> ACRPGATRMKWYFQKPYVRRVKSDFFRFPLLSQVTKQKIDWQYHHPRSGYEAACIFGPNTLEVTNLPMGKTCQYLQERLWRFFGKFGIVEQVRVLPHERDPYQTCGTAYVCFRSRMASLRAVRLPVHLPASLHNRVLHLRHLGTDRTSDDLFYFRRQQAISNLVAIAQQLYAYLEERGPLPAHRALRLLFERSYPRLAWRQAGVSVRTCCGSWLGFFSRSPFNELFYLAREDEVARPTEVTELEADPRASRKMISNEGTEGAAETRGRKTKSKLGDTKDGTSPGLKSLTDREENAMLEKMVIFPHLLSREKLQALLLRAGRLLQMDLQNELSVHWRTDRPPLPDWTQKQIQLWQHQDPLPEELQIWSRTKDYYKIHEERFLFKLKLKKERAQAKQEMKQQRRRLE;> GADHVFNIFKDLPDHKILEDKHYPAWLFTLDKPEKTYGELAMTFLYGVGIENATLDEYLRFTRLHTKNLIKLNNMRLKKSKRSSVKPLFWDA;> GGPGRALCTPTFHGLSDGPYRRLKFSLKPIRHDYRDVLVSADLRKLAETAQELLRGKETKRRAFWEIFSKRVKASAHMLSPSLMALIAKSFDVHDRDTGIYVALATVLPEAVKRADGRSLLTLSDVFSRRLKRDSNPHLFSTLARQLPNALYQLTGKDVLRILSSLDAAGLADMLACRQVARKLLAELDELDSVDLADASAVFASQGYRNPELYSALARRAVDVKDSFDAPTVFRLLSGFSQNAVACDELLESFSTLLVSSKDQFTQHER;> KNFKTDLIRMQWPAMRDEMVRFFQSQNAIAFDKISKRHPSASLSSDASSSSSSPSANRGERRATAEEVDREEQGKLSFAEMVVGSTRSACGVLGAGRSSAVDVACKPWKRFVRKEDIQRAGYVPCIVEKYGIERRLAIHRDTLEALAFDEQHGHLSYLFQARLFRLRIGNWIEECIPTFVQADPVARRLYFVKFERHVAGKISEVDIPTTMVGLLACPAYQRGYHVELVMPTIRCQCVGAEIPPPFFVDVSRLHYSPPYTAITLQDLQHLLPADGSARFHPSYDAATQEVAWAYEVGSLPDAPLPADYVDPNFVDRKGQKMDVCFRNHFPN;> PSPSSFPHYSRRHFKRQSPRQLHQLASNLAARGCTDVVLWSSMIQRAIEVNRSPESGAADVSVAPFRFFEALGFLGAVSSLGLTDRELFLSFVPCFLRSLSALEPRHLVQLLTVYEAAGVRPRGLYVAVFNRVLKLAPSFYSHEFADFLCCLARLKIANPSFLSAFSQTLVSRLPEIAFPDACRCVGALRSLGVAQQSLFDLFDERQKKELELLPTQLLLEDFQKVLSLEFSWQAYENMIQEEFIKRTEAMIDDKDVDELADPFACLNFMKTRNLVSDKFLLALSKWCRAAVNRPATRSYKRPLAHQLVELHDLMRERNLEQNKALEQAVLRFVADDGGCKRRPREVKPLLYQRNRRYISCPDLIPDGIEPARPCAEALPDVFMERQASLVRACTPEDLARQELPFAVQAETAYRRLQRNKRFLRFVQEE;> RWRPKKSYKKRTMGLPSTKARRRWAQMRRG;> GKRYIPFRTPRNPKSKHILATPPPLFAATALDARSFVWPPLHFVERRRRLLMEKNLL;> GLWRQSIVRCADNTGVIKACIIGIRNKYGTGKIGARIRVSVRDKTPECTAPKMPKGVIVRRRKETRRKDGSYIKFDENAFVIIQKNKARGTKIKGPVPMEIRHNCKTLARWIFA;> GWSKVVNFLNKGVQRRPHRRLPGQPHHQWNMLKTQLDQLVRSDRLELTLPRAHELQQYAEELVHFAKQNTPESSLIVESMIFTPAARRKLFHELCPLYANRPFFYTRVVNQHRLRMRDAAPMAYLEFVDRPGEIRPARPVGFERKQAIWEEMQATRRGRRQWWNHAKKLGLIDEETGDVISDINALRRPSAAEWEESDSEEEKADSPSPYKMVAAPKRALEPFFVDLPPPTERYRKQRYVFKRFRP;> MTTREYEEAFLPRRLKRIKVFNTPPPSELPAFFHKRLDNAHSNPRSILKLYRQYMRKDDYPAYDWLVRCFCHLGNVFGFNSFWATKDKQVIQALPSFKFLVYDLIERKHLIEARQVPRLLYAFACLEYRSWHLLPTLLEHVEANLEKWRTPTLANMALTLALLGVGDDAPDHNQFGPPDLLSRDYTGLVSKLALEVHRRLLALQSASSSGPRKSPLHDSLGCMPFDYAGLAFALTLQGSYDLCLPSDETAKSTLALFLQRACEPLSLEQLENSGWVQFFLYQTLYCVDVEKPKREVEVKKAVPFAFQKHLHLSWLDKILINAQPQGNELLQLDVDAALKRLHITDALINCSAGRQWDEQHCWFAGHLVRSRNLALEYDYLLPLGPGRPKVSGWLACKRRMLKAFGLNVATIHQSFWSLLNLEQKDVQLTRLLAQFPPVLEAVKDEKKAYEEDRHLRFQRHARQKFETWPPEKLEI;> SQSYPKGSFHEGHINPFADVQWISRPFMKRNMPRDHHPLAKQHTSLKAVTMLDEESGNHWHVLDGKGRSVGGLAAQVVRLLQGKHRVDFTPRTAAGDSVIVVNAIHLKMAGHTWDTKVYKFDRKTHPAGPKIITAKTIMARNPAMILNLAVKRMLPPNRLRPIMYRKLFVYAGALHPHWQVPQVIVPAKTPAEVSFLPFSVERADPVQAAARIAALG;> MQIPRDVIFEVVRGFRGRSRNCIKIARVRAMKALLYSYIMRRQRQRRYRVFWIGRINAAGREWSFPYAWLATSLWRQNIWLDRKMLANLAETEPASFRALVNEGKSVYFWNPDKVRDIQDL;> VRPNQGRNDYNQVGGKKRGQGVQVLPETIRLLIETRKAATAGGPVGRQPLPKATEATGVSSWGRDRRFPITEALRLPTVAEVNAPWEPYDETANKRRSGSRPLSSSVDGCHENHDPSSDGVARGQDRLGRLDKVVLHSGDISRLRVDATVVGAVRSFKTVGDGRGFTGCSALLEGAGPFLSSFVSQQRRHLGEELLHTPVRGDPSSAQTVAAAAVRGLRRGIHHFTASTVPLPLRSSSTVPSLAEVEEMPIMELSQLAARAALLGSARGGGTRGFGLSSHPQTRRLEGVSTASGATEGSDAALSFANEVRDQATASQFPARDLIQTPLDPSQLSPPGAVLISPGFNLPSNFLIHVAEPNAVLSNQQMLDTLFRLEEREALRRKEQLLSRFGAAQAADEAMSDDEVREEDNEMTPRSMWQDDAERDTGVQRMLLLEECYINALNAAWALGVRSVALPCLGAGVGRFPVYIAARCAARGVARWMSEHRDCDAWENAESDKRADFDRIVFCTSSDVEWNALRRVIPQFLS;> GTSRRLSLFFSDPPPAYALSLHAGYKIQAALCVDRLPLVYREPRYEKRWREFKEQWEAQTKNGLTLADEITFMKFPFHFFETEEAQKKREELISKTGDAEVSELELLLSEEGFSGKRKLQRDRDAKKAAREEQSAVKSAGRGQDEKGLRSLEREPERTLYLIVRYGDSWQFPLEDRIHGQSMRSTLKRLCSEQLGSSYAPFLLGYSPFSYAKRTYPKKTKEAGILGRKIFYYRAHHIPGSENLKLPEGSPVSDFAWVTLQELPAYISPRKLAAVSAGLLLEE;> RWWTRASGMRNPVKWTRDWEVLNRKVYFAFDEREIRRSMLDAVNAHRKTASLFHRMINAVPGVAHAMSLPGPHTFFLPSDKACRDHLSPDSLHALTERVAFLEEQQRQRVGARVQVEGGVSVRGGTAAAIADRVAKTTEQLRTFVLAHLIPGEWRMKTLLLACGAGDPRRNGSLRYQDTDRELFAPVMYASRLGTGEKTKRRQTASREGVEHENAQELGRTRDEETDRSSVFLLPPPQSTDEPLPVWVQASRYAAFLPITTSTNFPRFEGTECRGNSDREEAESVENSGEYSQRRSTVGGALHLWVGGALVTKGDLRAHNGVVHMIDKPLIPVQLLAS;> WHRGTLSLLCSSCRYVVRKWHVPILGVDCNANPRHKQALSVPAPRSRGIPKHLYPFLVGKQYPRHPRWRQAFTHRSRMGKYKPQVARN;> SANPYKPKSREVFHPYVPAPEHLPPPAYTTAVLKPMQQFIPKDFYRDMRVDSLRDGVSLGSDFPWNVTHKYRFWRRRKYNIQLDDRFIRLSPVTGVDYYPRLNVFAVQWREDGQHRIRWFRAAYGLTRAMRAAENFRKTLEATGRVDN;> AISHLNPSISKGKVHYRVPNPYIPVLLLQAVPGLGKRGELKQVRRGTLRLFLAPKGLAVVASWQNIDAFYLAEKEEEERRRRAQAGR;> AKVGPSKGRGPLLAKFAPVGFKKGFGAIGLGRHTKKGFFIINTMLVPMFKVPDLSNCKLKCYVAPDTYRIVQQSFNKRE;> GILRPRERLLLNALKKEADIRYRGRRMHKRFRSWAQQRVRHYWLPQKVCVTSDPQLMDGSYIAACVQKAATLRKHDLQLWHGFSKRILELADSLTPQQMGYIFYGYGKSLFRHEELYRGLLPFVAEALPEFHSHALMTVAWALERVRVNDRAVVAQIAEEALAKKDLMRPADFIKIVNCVARMGAAPPSLAAALSAELMRVLDEKCNALLFRGAVDHVAVATLYSDPLRLYLLERFTKTAICCRPMHYQKAFQSAVAIRVLHPPVWQQLSKAVRNFYIRLSLRRIPQRARRPSPLHWDVSNALAKLGVFHRNTFQWGCFWIDIGEIDDRRQCWFVDGPSDFYSSTNEYTEANKLQHRILSELGWNIRRVRWNDWVQLGTDMDAKVEYLRKLRERPPWPAILTDGPSSSRQEMVANLRSARDVQRALKERREKNRQPHSLVMNL;> SGALQRAVREIPWKSRQDILRERERPVYAAECRGTPRREYSKNVIDGVRVKPTFNPFVKLNKAKRYVLDNWPSRNWDDWSPYRCYVRGSRRRYNIPQDLLPYKDELGEWHPPRLSARYQADVKKQYLMNNLPWVWQKDFYEGKMHFGDREPLGPKVWYRKAFREERVKEAMRKMDDLVLDYRQENRDRRRYNWFEKVVHDFAGEEIATQFIRKRKEPKL;> IATLVERSLEKHKDRLFDCGASGQPVTYKEVAEHARSISETLKAAAAYLHVPLTLPSALGRAGADGQARHTATSTEDCTGSASTLKCRGKPLNRPTIGLIVPPNSVAILAHLVGVWQCGGVGLLLPFPDPACLPFVADSTAAAAASAANAAVLFAKGGKTLHTYRPDALFQGNTGPSVYAKTVNPNSLPFLNSQNNAHNRNGVAQLWEYQAAESRCHLLVVTPEVAPMAAEVASKLSIPICVLRTSWVRKSDGTNGAEEQRAPERDLWSVRGRNKLEVKAYVPEVFHDSSRTSRNITRWQLLEVTPHECTHAAADEESIAEVAAPATHFFQGPAAHAPRAVIYSHKALSDQVIRNKDLLQLNAEDHVVILHLPFFGSHRSGTGSQASSRMLCTPKGLVAVAMPAVAAGSTLSFLSSSDKIQDSLLPLPLQLQRLQDRLPQNEKIPRQPEQRQALLPLGCDIPEKTPWRCSGTTTRGPLVPRGNQEGLQVDFTGAYENTLEVNALQMWEKIASLHEDGRNTTRSRKQRFTSRDKATPELSRQATVLAMDAETAATMVQVIATERFQMEGTNEKAHASGGSDASRFPTITSKDITRYKAAVKSLRLICICTDEGDLGASFSGRWSSSNKGGGIRIQSLLRSLQALAGPDTKILHLCSLTETGLLMVGGPLPDGSPGSRERGEKSDFGEPLQDHLSTGCKDSKTQCLDATDGEDRANFTGVVAPGIKVEIDDETDQLRVRSGHMAMGFHGRPRSTQESFDSAGLFRSSFGGSLVTNRRNDTDIIGCDRGEAEQRVELFKCVYSAAVPRLPLLHRLIASFKNSPKMESHIEGYVKKKPIAGRDWNNLHAPRKHWKKMFL;> SVVGRFRLIVPAATAKPSPAIGQTLGPLGINMMQFCKEFNARTANVRPEVPLQVTIVPLTDRSYKFSIRAPSNIWFLLRTARCPMGSESPGHQSVGNVTLKEIYHIARCKSMDWPLIGMSLRGICRSLIGTARASGIEISKEILPAYHKRDYTDVQALDSMRKDMRQRKKAAKRAAT;> YKPVIDWVKNRINARMRQYRKRSLKKKNHSKVIQRFKLTRFGWQRLRSGRNGEKENLTHKQLKRTMGYTFVSRDDLWKFRFQLPSHILRLRDAPINRNPNIRKIRRSLPSYFG;> MLWLAATHRNRVAFQLFATPREPTASKAAAAARAAAEAVARSSTVSAPFTVQKQQRLLALLAASSSVADPSADLFRVHGLPGFSGFRPSSPPHLSKLFRGRVSRHLSCRRVNHLGRNNSGRITVRFRGAGHFRRLRFVDYKRGRKDIFGTVLRLEYDPNRSAHLALLQYDDGVLSYILATEVTRPGDRVVASKHASIAPGNCLPLGNIPVSTIVHNVELRPGAGGQIVRAGGCYATVVAKDRHFVTLKLSSTEVRRFPADCWATVGQVSNAAHAERIRGKAGVSYWMGERPRTRGKAMNPVDHPHGGGTGKKGLKRPPVSKWGILCKGYKTRAKKKPLGLIVRR;> LPNPLVHLDISIGGRDAGRMVFQLFADTHPITAENFRCLCTGETGLGYWMRPRWYKSTPFHRIVPGFMCQGGDIHRGDGRGGECIYGQFFRDERFLYKHSKRGLLSMAKARRQHTNNSQFFITFDACPWLDGEHVVFGQLQSGAEVLDQIEEQGTPGGWRKRPVEIWNCGELLLNTLREIPREAPAAVRHQEMLKDLIIDATERPEKLYEPSEQVIPIPDDVYIKARRGF;> NKVRTDKKERKRAFPQRGFWKKQNFLQVKNNTVRLAFAVQGVDLLKLKRLRWGEVRKGNTGWWTDDYRSP;> IADRVRTSWTYRHSRYSGGVRFSLPRFMVTKRTYLSTKFRRPSTVTKWGNPQYTLPSNVQREMQENSAEGDTDQATSEELGGRTGKKELGRNGKSAGKTKKAADTAAQEVQHTPKYCDMLFLHQEDQQSRRR;> SRYVKVYRKVMNLQRRKTPLPWTPTFLEFSKEPSVPFPVREKLQPAPIDLSYYLNMEVGDLVEVLHGPDCGRQGVVLSISKKRNTVVVDGCNMKKSFWNPGVGASLITQEMPIHITNVALLDPVVKRPTRVKRRFMMNGECVRISKLSGSAMPEPVSTSALRQPNLYQEYLRQKALGPPLKASYARPDPLHLKILQRLARHISWGQGSPLPTAENPRVNSPEPMALRR;> RSRSKRLFVQLKSAAMTNFCYVTRKSPEKKNFRIALRKYDPGVNKHVMFYEARLPSEKNKKQITLSLQRYIRWTGKQVKLLLDKVEKAWEYGRFQKYFDNQAPLLTDRRGRAVPRYK;> SHVPYKVVRTPSGNLPVYSRVRKHGTEVTTIVRHAFGDITAMKKDLVAICEAPVRERLGTLEVKGLHVLKIKQWLRSLG;> SVASRIHFLNSRTRFQTAVHASDVAPPFLLLPLASPRPLLAYHHRFRTRNRKRGSRFHPHPLPLPPPPLSPPRSDAAHLFAGKPLAASAVSTAAGQQTLPPPLLRHLQGLFPVFRGPECDPSCGVGPAGEAAGLALLPPPSLVEPRHLEDLARRALQARGETRDAASGACKSDRLFWRELAARVEKVRDLLPIESLVRLLTILTLNGASGTVRPVKQIFQAFETQDEDTPATPANRTGLRLASETLPCVRPLPPRLLLASTREFLEDLKKLSPPATAALAATFAWSNCASSALLFALMERWAWRQPRAEPSVQTDVESEVEPLGKRREAETGVEEEAENAKKLEAVETQGHLGDFTPADFALFVSALGHLLSQQEATHVKYSRQARHLREISGKQIMAAFREQKRQKGKQTADANFENFEETKSAWHFTAAFFDGCCRFMATRAESFSLFSFASAARTLVENLDAVALVGEAAESRALAVDGEGAGSVESLGIHGISTFSSFEGSVSRSEKPHVACPTPDSVEALAKAISLFVASWDGGDKTHGRLATRAANLLLVARLLRAASQCELYIHLHRALRLEAEGSGEGKSPQKRNSGEQASGAGVDDGGRGIAVDTVGACKTLLEHISCELGLLHSELEALPLLNSTLEDADDSADEKKAVDAPTERGFVHISPDTVYVRNELLAAAGESAAAVVRLHHAKSLLQATDEVARDSQSLRKGEAENVCHLSTGARVDRVKRWMRGQQAERMQLETLGELKSEAEHLADAIDRVLRERGAAGLPTEQLADLMEVFALCVGDKRVSQTPEETSRWFRLGLGDKAEKMNQANLSSLQALSSEIVRRYAALDVNQKRRIKWATRQMDWKDPYLNHCLGRFTAAVTRQR;> YDSRWVKRLDRLRESKFYDPAPIIKEEEILEADKIHPLLKKVTPSWNSRRTGLLAYKIGMMSLWDGWGERHAVTVCQVDRCVVMDQRTLDKDGYEACVMGIGYKPIHKVTKPMLGVYIRSQIEPKSRIAEFKCSSDCLLPVGHEMSVRHFTPGQQVFVSGWSKDKGYLGVKKRWGFAGQNASHGVEAKAHSSPGSIGQSKTVNVVWRFKKMAGHAGGDPRVVNCKVFRIEAQRNLIFLKGCVPGYKGSLIKISDARGKTHHRHNRHIPLHFPTFVPEPGVSYPVTLECPDAEQDPFLYPEIAIADK;> YWPPTRKDRSKRIRLPSGKKCFVFNAKRDQDGELEPVLCFVDSQDNLLMWFNEEELLEFEKLMPRLESYYELWEEKASRTRMKEAIVAEAES;> SSGLPNTKRRIRDPFWRRSGWWRWRQQEVKAMNRSRAFRRHLFPRFTTETVSFVDAAEAEAKRFKEIVAETGRYPGQTVNFFVPKVEGAKLDPFAALPSRQKRLKLRRKAVREAEEAEKAREDADFVWRGKGGGRVWEERKANIPLGKKKLLLYCTIIKGLQITDAIDWLSSLCLHRVNYLLNLLNASRKKIHEQGGDISRVYVESYMLNIQGQIKRPQFRLRMVNLIKTWKFAVVLRFREYPMDEYFHKLFILKHVPRSLTTDMRLALAGQRVGLHAVRDWYPFLDSKTRFFHRKRLKWLDRTRQFDYCLARRVFKSKYEENCRRRKIQVLQARGASDAVIEEAN;> GNFRIKPPGARHAFPKLGTHRMVMFRRMNLLNWPPEDASPLHPIEPWGRQFFVFNAFATIDPADWCGPRGPFPRLPPLAKPAPDAATLAASPSSLLSALRETEERSATRTVMCVTDFAQRPLMFLGKDDFRALRENLPRIKEELKAFKERIQPNPVHAQYDLRRKLLVYPRQAMQRLKTGEHGGYGTRRGTIRERKT;> PPKTPRNVFFPWQVFSVHRTGAFLERRRVALKVPVNLTKFEIQSYLEKIYGARVLKVSTLIVVPRRRRDIFGPRPSMRYYRVGCTFKKAIVTLEDGVPDAVKMLRSSIELAKNPDITKHNLTYSGRVRAFKPPSAAQRWEMGESKYAWRLPIPNLLAGDEMQLNPALRIDESTTQMFPDFSKPFFHNAHFNFSWKPEEVPFQQTVKLDITPWRR;> FFYYRFHKRIGKGNFNRYLEFYQKPRGIENTLRLRYNYTPTFTAKKRSEMWKVNLVKKIAHATDAKQVLDVWTYYRHRRTKRPYHYLLALQRLVEVGGCDPTDFRFRLIARGIYRTAKRFINLPRVCVYLAKLNATGDLQDLSRFLIPQVEAYFPFQLCLLAHAFGSVRLQDKVLFAAIDEALRPHLSELPAAMLVKLTQGYAGALVHNYGLLARVSLLLQQRLSRAATGEADPLTACDEEDETGRTLSSKEPQGGSRQRETTKAAREITEAEDDCLEATEKKTVKRRHSGPLLPTLHHLLAFGRVCADLKYQDFGYLEMLSIQMQAAFRADLAVSSSRETFQRFSPFSVQELVEIFHRLKVNDVSLLLAALRHVQARMHDYPPSCVASIGFCTAQMLPCDASTVRQVHAQMLEVLQEAVPLLDLCSLGQLAAFAKKAKPRRNRSALRSSVFEAVEARVIELQGDGRTVFDVGRLLELLSLNGRRVSEEAFHILCRQAHRHLDLFEPQDFCRLARALARVKCQGSRGEQSEGLQASSLVNALARRTLRQEDEFSPRDFLSLLRSLTLAGPPDRVYAVPLKEKLRRKQVLHNYFPASQSEDAEAFEDSEQLLESDLPPSSRQTPTLRKGRLLLGPQVIRRPQQQGSPESAEGEARSEKETLEEESLSYSPVPDGEQEAEVNGNHAGKSVSVLSEGGRSRIRRRRLEEKLRIAEEEGWDLLHRRVASLRQLKGWL;> EKLYGIPHNGFWNQRRMYTEARGQTAALAAMQDPVEVLNFAGSNEMASTYLLVSCLRRVSALCDKKHAVLETVAKDERLQRLIQLISPHVDDCDARCLVDLCWAVWGFRGAPDVVEPLLNRMASVVVRRENAFTPKQLGTIAFTFSWFRGAPTDTVADFVLAECVKLLPEMEPFHVTLLFGSLRRMRRLNRDVANLMIEKLTDDIDRFTSDDVVGVLRALAANSITRGFLLRRVATLVFDNLDSFKPKQLASVLNSLTLLRFLTVENGEELFSCLSGSLSELPAASIAEILEALTILNFPRPEVVRTCLDLLAEKNGLISQGSWVRDHMIIAAHAVIQFQLYDKNPVVKPLLEELFRSRVNSSRTQHRVEEVIHALDLEKASPRVDVPPYWRAMIDQANREEQARLEHSGLQNELTLVLDSLRGKFQLQIQKNQQAGPYSVQFLDDETKICIEIDYPCCRTPHIIKARHLKQLGYHYLLVDCWQWRRLRSEAEQTVFLKQLLSGPLLEVGRL;> RLQRLIQLISPHVDDCDARCLVDLCWAVWGFRGAPDVVEPLLNRMASVVVRRENAFTPKQLGTIAFTFSWFRGAPTDTVADFVLAECVKLLPEMEPFHVTLLFGSLRRMRRLNRDVANLMIEKLTDDIDRFTSDDVVGVLRALAANSITRGFLLRRVATLVFDNLDSFKPKQLASVLNSLTLLRFLTVENGEELFSCLSGSLSELPAASIAEILEALTILNFPRPEVVRTCLDLLAEKNGLISQGSWVRDHMIIAAHAVIQFQLYDKNPVVKPLLEELFRSRVNSSRTQHRVEEVIHALDLEKASPRVDVPPYWRAMIDQANREEQARLEHSGLQNELTLVLDSLRGKFQLQIQKNQQAGPYSVQFLDDETKICIEIDYPCCRTPHIIKARHLKQLGYHYLLVDCWQWRRLRSEAEQTVFLKQLLSGPLLEVGRLEG;> RELGLGAASAIEQKASAFFSRLTDVQQRQLEKQGLLASRFYRFLVISLMEKEGTFTYYDFYVWRKGCLAYLKAAEEEMQGIVGKSARKLADLGWEKLRPSTSPEFKEMELHLKILSHFTPEELSRDTAEQFTSAAIKNIAKAAETSVKNVKNVLLGHAIALTDRTWYMRLMEMQRPIPQSVEDYLLLAETDRPYMIRLPYGEKFYNYELEEALAKKRASERHKSQRDVPRLGRKQHRIRRLFVPNARVAFDRWARIPHARLDAYGNFLYRLNQPAKGAAAVARAAEREKLRVEMSENAEFYSDAALSASRITLNNLPPGAFRRRTGMQRKSGEIHHVAPPRDPVLRELFAAAIQREKDEKRNRERRAQEDAAAAEK;> GGSYGYDAFFRGAAEVLNGSNIQLPHLPENEEQKEGKVYQLHSVRFPPQVRRLGANYFFRRQRAVPLTYYHHLVEAKPASEGSAPDGVHAQTGRGQALCFVASANPGYLQSKELENAVFESTRGFACQLILEGRGVKAYFDPEWPNLMVRLGVGVKPLALRRLAEQYATRAKIFVDKRGLLLTVHGYDKCAVGTLAMSLFNHLQANPYTMKGAHVAMHPIKKKVTR;> GIDELWKGSYLDPTIGAKQKEANAVAGDAWPACLLRMKSFEDLHKLWYICLKEKNLLMGERWAARQHKQEMKQPERLQKVRRTMRRILIVLTKREIQQQCLRAKDILAKQQKREALETRRFQLEEKMLQLEHRIRRMEPAQSLQKEAWQATLDRYRSDHEDILIQLHPLRKETTQLLAPDWRYERKYSDLPGPIRWKKQYIPALEDQYRKPIRF;> PLQPSFTPSVAFPAHKPVPLNSPLSPSVHAAPQVRRPGSVVRMNEVIRHWWSVPAVGFNSVLEVPIYRFEVFQRRAEEAGEGEASIAEEGDHPEEEEGCVVLPNDIFGLPLRPDILYRCYWFYRRAIAGWTERMQLFKWEWPGSKRKLRTQQRSGRARIGWRKAPGKYVGVKAHPLRPHDQRIKINKRLLWQGLKIMLSAKFAQGQITVVDHFNLQSHKTKHCVRHLRRLLGRKCPSALLVHEGTTDVNDNFRYATAHILAVRRENVEGINVYNLLKYRQLVITEKALLKLIYNIQTYPEKRGWLPKYATPDGKPAPAPEKVEGWDREWRQMKERERNAKFSKALLRERILKWKWSDETKGAIKVPRVDPFKGFRLARFSLHEPTMPWEKFEENYVDTDPLEDEEDGDMFDEAQALGEETQRLERLDHEELSDAAAYDDMSLTDMPLTERMHRPKRLENFKMEP;> SRSFPLGIKQTLPRHILRATGDQPSSSSSMSALAAKPPKSPCSLSVDTCKDSSPSELVVYERRDGKRWVHRHQLSLYLSHAVGLGYFRAQFEDSSVTPAAVFDCLSHLVRPPVHAARSEEDEGDEGGERRQNKQVDGAPDGDGERVTAQDLSEFMKNCVASRYRDVDVLDVVTDVLSALLIGSADLPLLVDIASSCIALSLLRPKLFTAIASRLLVLLPPAPASGSSPLDAAALSPRQAVRLVESFSHQRFRHPDVLPLLFLSLSPSLPFLSPRLACRLLHAVAGLGACAAPAETVQLLLSRVASGLGDCVGRPGCESETHCQTATGDHRMIQQTSDLPESEFLEKQIQGQKLQPQLALADLTKATHALLLLEIELEQKPLLESLLTAMAPEIFDHPVEFWSSSPAGPSLHRRLLLIRTALRHLHRDTIYNSLPTMVRQAFRRLHRIEITSPPRSPTHFVTRMSALLTRLRIAHFCYAIRGPLVFDVLERDRPIVWQCNTADRFYVNSAEKTTAVKLQERITQAMGLKVGNCEYWQWMKMKRKRTRLEYIRMQRYYILKDRRQHDPDFEGWTLPLVHHMHRRNRLHYDYYFPNYTPLSRVEY;> GVLRSLYSRVSQRVWSTLHFRVGSRGQVRTNKGFKPTAFPHLGAALFFARMSKGLTRDSVEKFVRLNVSEAQRQEIKNWPGSVVRCIENGACIPSRELQSRLEQVVGVPLTRRKKRAGNRRL;> EPKVYRQREGMIQFVFQWGIGNSFRAVSANRFRPVHAARPKEVSIHPSYFESPHPFVIWEPLNEAWEVYFYENLKKSAKPFPVKKFGIARAKREALLFLEQMKLEGKLEKPTFSSGVDGVTFDQVTGSWICRFVDEEGRCVSRGFGADFHGFEEARKLAIERQAEMKKVEASGLGPRMRLVKEK;> MASRGGTLWHLKEVVIQYSASGNSSQGLRFFFRHLLHRWKQRNPQVQVHTVENKYEAPKATFKYLGERTDSRCETPLKDLSPGQIEQILDLHRNSKGDNRFLKHGGPRTWTERRSIQGLWRPSLPSQLIALKWFRRKRPPMRLPKYSPLSLSLSIQAIRGHGRWGSEREFPRGWDQLHLKDILGSPLRSE;> MKFVHPRHWILQWKIRPGDKVVVISGKFKTIRGTVLQIDKMRNGVSVSGVKEQKRVKQEDGSFIRIPGLIHVSNVMLIDQAIDLPTRVALRVDDRGNVVRISKKSGLVIPWPNGEMIKFGDNRKSREFLKSKEERDVELRKEQNDDEERAGPKDTPAEVAVERTYDYQRDVATMQALRQMMTKYNRDFR;> NESSPLHMGAGSANWTAVARLEDFTLRGLSHPPWIHVSSRPFYGAGGGAVLAACMSSAVW;> PFKIFKASPPPAPTGRKPTGYRGNHWHKKVLYDPVYPTTKVPAALVPRYPIDWRNGGRALLIAALSKLEGASALQRRIFLRENSRESQVPQTPLSPFQTGSSASGGGAYLVSSLGRKRSYVGRIAVSLMPRHRQIADYQRVGGFCSPRCFSECSKELRRCLCAWRCTGFHEHVVQMDGMLGEYKGEVKTEKPLFSVLRRQARRNADPSEGVAFCAESAKFKSVRRAQHPAFEAFDRQGPDGPSQKPAPRKEPPLPFYSASHVPNVPRPPPPQPYTGPLKVREG;> LRHRVLPSSLPNRLFSVDNRETTRFWPPPLQKEEDERRGAFVESCLQPSGKASLLQPPQCLPRAPSHLAKLMEEEERLRLYRHLKKEERDAATLNKFGIWAGEPIADTPAAKMQPLVARTCRQTMRHLQQIEIERLDKQRNFQVPLFGPGDLMEVKYELSRSQQTFATFQGYCVEVRKKRLNSSFVLRNSYEGIGVEQRIPLYSPRIISLKVVSSCASPTQDFLLERHKPLTRDYRYKWKYNFRGRWSRRIGKHKPGIRSVEKKIRQRIVRIRKRYMGQRIEAGLPPYVWGGPYPQYGRKRSLFIRGEMYRRMLIYSFDERRRRAEKLRKRRQAVKWGVFKLRQPSVPPALTALPTYHPLYPGNLPKR;> WYTPPSKRTWSKQHNKIFTPRPLSERFSPHKLHPEFEWWRERTVQPSALFMGFPDLLALPLRGGSAYIHEMDAATLAVVLASLAHSPSAYSVSERRPPPSPSPAVSLSSSSFSPTHLPQHLDSLLALLGRQAAATAAHAPDSTLAFLFRGCAEAGVVEKNVVCTLLGRVEQRLPCMQLPECLVLLDALRPGLPEVYRHPRFVARLVAHAGLLLQFRGAESEAEDLCDLAFSLVFAANCRDAALLQTTALLLVHGKRMQSLNETAPLALARAMEAFAACRDAVNAPLLAETAAAAENGDAEGSRNTKAAELFCASPLLRAREPSVHLSPSGWLLLSLLSPVVQALHRAEKGRRKRRGFHQDGEAAGLTAEREVQNRGASRESHALTEAAARAAAAVAEETQTLKNRESSLFRGLLRCLERVDDHRESLSPGSMCKVLFAATVARAAPSRDFFPDVLKRLGDQLGACTPEDLSRALFALVKLSSVSGLDPRCQDLLPPLLGTVLQAVESSLPVADVASLARLHSAAVSALISSSETKKEEMKQLAEETSRLMHARLEEASPAHLTAFVRHWDLVPAPSGAFREALVAQAIRQLYFFDEDHLSRLLEGVTRLAASSKDETLLASVDELFRRAEEEATTEQAFFSPESCLRIFVSLVRYGEVRPEAPRNRERLVVALCNYLTGVDSVAAVSSDGASDPEELWVKEDEDLPLLFFAEDAKGFSLREDSALDRDSANESRLQALSAASYIRLLGALRELGVRGGVLLSRVAQLLHMKRYDLTDAQQEAAAEIC;> PKNLNLWGKYLRLVGRGARRGFKKWQVIPPIPVKAYGREPSAASQTGLYHDEDFNYHTKRTFSMRRTRRKIKPNVFRRTFTSSLLNVTIPNVRVTTSALHAMDDMGGFDAYILRTPPQELRSHMGERMRQVMYYYQDQPAIRDWGLPWKVFLKVASRRDPFYACYRHNLRKQQYEADLRSRVRSFSPYYLPSGHQPHAERQVFHEGAGESPPLNLWWRENRELEEAFRRRLGEAKCFERAFADSSEPLGYTKGRCRGGGGKSGRSVRRRSKTHKYRENRAF;> NAERGDADGGTSALRVTREQFHDGSRGLFRPHPFNRRFARVRKPVFPIEARNLRLMYKRKSKRRRGRGDKSNAKGIRWKHVHQQAGRYKGPRSRTFEGGKLPLYRRIPKWPDAWLARQRKVLEPLNLAKLRTFIESGRLDTRFTITQRHLNDSRCVKVKNGVSLFNVNDYPFPYKISIEVAGADQSSIDAIRRVGGEVIIVYRNRLNLRAHIKPYKFEVLPKTARPNLEMVHYLEKMRARGCVVKYVKPQWLIDEEKSLKTELAEFEAEALIAKGEAIERGDPDLRESVDDLQQRLLKRFRLRETRAAELL;> PKHLTRYLPFVPTSLVHETTSFLHDATKLRALLALIFSPCKPEASVADELASPAARLEFQQEKERYHAIRDQHTDCYRRHESAAAASMWRAIEALPSDLYEEAVQSVTFAPPYENEPPPPDPSELRPGKNASTETQAASAGQQPSAASRGSSVRTLAGPGAAGEAVSQPEHGFYHERFAFPRALMFHEMYGEQIFQSLSQLERRKLQVFMNLMHVRYPHAELKRDKPALFWLPERQVLSR;> DRFRSAVHREMIVAMTRTHLQNLLLKRFGTFKTQECRILASPAFSAVVLKAWASAVVDANLRLDGEGAMRLAYASPPPAVLSDPKVKELVASDPEAAWMLKKLSCQSVASFASLPREEEALEEVVRVKQKDNVPQPHFPSVLKMDHPQFPYEPHELEKMRDLYGVLLKWPYREQGQVASVAARRASLESKREERLRKGETEVAGQLKVTTGCSDSYVYAPSEMETGLYREHA;> MRNAIFPRIDFLRYLKKIHVSYCPTRPKTEIAKQLIMRVTSESVKKKFPHLQASWEMLAYDAPATVEVELLDGRRVRRIIDGYSKAEKKKIVDDWRFTANMEPWPEVLGPQP;> PPFRFKAPQEVRIKVPIGRIPPAVGPEIRLGKSIVAVAPHRVTAEQLEDARRVLRRVLGRSKEVHQNVHATYAVTRKPEGTKMGQGKGSIDRFVARVPAGRILFHIPQINPFHPFPEVEPNFAAFKAIAPRLPVPVVFREQNNFFQMHSVKDLIRKRQAEERENREKTARDKLGGFHTD;> TVKSLAAAEQWEPSPLTLKQHQQVVVWKKDRTCILCKKEVQGGNVEKVETACEKAWRFLSGYSRSAHVCPILPQMRILRYGELPLRDRAKFDAKLRRE;> LQIYPQRRVIGHRIEIFRGKHRRRRMVPPRIPLHPLAANTSEETASKDMNLFETYRDLQLRWKKTCRQRKKKFNIARKWRMPRNIRPLPDPSWTLVFHVNPRSGYRRGRGVCRDRRRENLQGDALEVSAEDEENRLAGKAPSNRDQEDRQRGRGAQETYFRSGAALDAAIEEENILQILARHPEKGRVEGSGRPRGADGWGRDGPLPQWMQILQRTPQEELFCVMKSNVSTQHKVTAGDLIQAEKLHRKQAGDKVVFGTVMLVGSRDWTIIGKPTVPFAKVEATVEEQTLAGETLSFFYRKSRRVSRFRRIRHCVTMLRIDRIVVDPNMTVDPPAPKPDRLLDLWANRWLYPDELDGIKRNESGEPVVSEIYDGREHQKGSYQRRGLTASYRWYPDPQSAHWRP;> TEPISHMQEKPATLRLRGLPYRTTAEDIANFFEGYSLAGPPDEAIQLHRRMDGRPTGWASVYFESEQEARRAKQDKHRSYLHGRYIEIFINFETGELEWIHQPQLSENVNRKHHGKDNRG;> GHKHSESVLQQFYNRLPVRKRFLKAIRKGTLIWDKGQVKIPPIAMQGYGLPNKLVLPHQKEFNNKLPKFKGKINQLKATRIWFQD;> ASYRRPSRASPTGQARKPHVGVRRLAAEYVWPGVVLVKQRKVIAFNVETKRRNRHFKLYPGENVKVSKVTNLVALCHGRVKFTHDVSRDVLVVNVLPERREELLREDLWRYRTEHVRSMEENRHICFLRRKAVRMFGKELVNPPTKPPLRPFYFTKYDSWENPALPDVPQLDDD;> AHKFAAPPCPNLLLLRKTIHQRLQPILFFLKNDVTMGNYVYDQHFKGVLCSPLFEGKSYKEIYAMVDRVLEDIGLSGRVKLYCEPPSLLHKMKYHVRKHWPLEKG;> IRPRKKGMRLDRRRSKKQYKHGRHVGGWNYRWLGS;> PKYDLFKPLDFLACVKSVHVAYHPGRPRSEVCRQLIHHMKSDSVRKRFPSLQASYQLLGYNAPSTIKIELINGKKHEFQAEHFSLREMQMRFDTDQFEAYLEYMKSQSVEAKP;> AVPKGKRSKHKCKQRQLIYFFDQFDGVFKRRRESFYRSFYNPPYFSKQTEQTSLPPSVLRPFRFPGFWPGRFAFKMAS;> GTQRVVQKRRHQMRILHPAQTAYVPVEQRPPPIPHSLTASSTVKRLLNNNTVAAKEAAKRINWGAYISHQRGVRWHPQGAWRVQFSRRNHERNFFVRCECYFRVGTYGFQMAKDLAIRYRQRLEKEWEELQEQWTKLDILEAEQRAKYKEKREEHLLL;> CNPQQTRRKQQYASIIGKQGLSKKQCGIFWDYYKRKCKKRRSTKKFI;> WNRNPSARYPKKGNKGCRPVCRAMRKIRKRLRTGR

Our study reveals how Toxoplasma gondii assembles over 40 mt-rRNA fragments using exclusively nuclear-encoded mitoribosomal proteins and three lineage-specific families of RNA-binding proteins. Cryo-EM analysis of the mitoribosome structure demonstrates how these AP2 proteins function as RNA binders to maintain mitoribosome integrity. The mitoribosome is also decorated with members of lineage-specific RNA-binding proteins belonging to RAP (RNA-binding domain abundant in Apicomplexa) proteins and HPR (heptatricopeptide repeat) families, highlighting the unique adaptations of these parasites. Our results reveal the structure and composition of the most fragmented rRNA mitoribosome to date.

The samples were fractionated by sucrose gradient, and the fractions corresponding to mt-LSU and monosome complexes were combined and their cryo-EM structures resolved. The LSU was resolved to 2.89 Å, and the entire mitoribosome was locally refined to three bodies, the SSU head, the SSU body and the LSU, at resolutions of 3.6 Å, 3.29 Å and 3.11 Å, respectively. As for the LSU rRNA fragments, the peptidyl transferase center (PTC) region is nearly strictly conserved compared to any ribosome and is recapitulated by LSUD/E the center piece of the LSU, engaged in base-pairing interactions with RNA3, LSUF/G, RNA13, RNA1 and SSUF. While RNA domains II and III are largely reduced, with a dozen helices, compared to the bacterial counterpart, domains IV and V are mostly conserved where the rRNA fragments recapitulate most of the conserved helices, and Domains I and VI appear highly fragmented but most of the key features are retained. The CP consists of the conserved mitoribosomal proteins mL40, mL46, mL59/64, which are found in other species, as well as Myzozoa-specific mtRPs mL155, mL163, mL173, and mtAP2-3. Despite the lack of a 5S rRNA, the 5’ of RNA29 extends out and towards the top of the CP and is tightly embedded in several ribosomal proteins, mainly mL40. The remaining three mtAP2s (mtAP2-2 to mtAP2-4) are positioned on the LSU: one at the central protuberance, another above the nascent peptide channel exit on the solvent side, and the third below the PTC on the inter-subunit side. The mtAP2-3 is located at the CP and directly interacts with the 3’ ends of RNA13 and RNA29 and the 5’ end of RNA38. Finally, the L1-stalk rRNA, invariably formed by helices 76, 77 and 78 could not be mapped to any rRNA fragments in our structure, as the position of L1-stalk remains completely unoccupied by any rRNA or protein structure.> ANGNEGLSTTTKYIFVPIATIGCGKTTVFNTLNNLFPQWTHIQNNNISKKAKLKICDLTLLALEDDDQSVVLFDRNNSASRERRQIFTTIDQK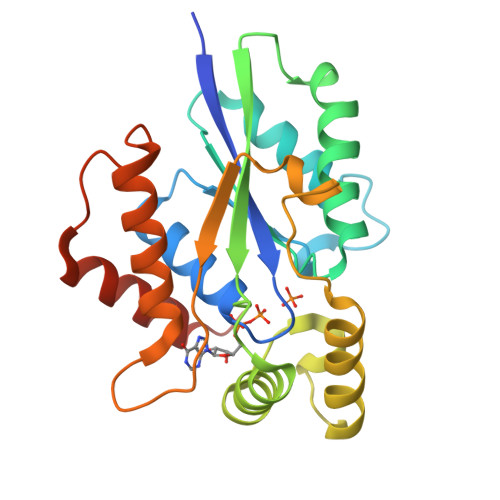RDEHLDDTVDLKYIAINFIPEDLSEEELWDITYNRVIQRGDNHQSIKSQLDENLVESVMKGFIQRYQPINTSRSPDDQFDHVIHLKLSKDENSLKSSLENVRIIIDDLVQNFPDLIKEKPADELINECFQKALDYKPTFVKN> MTTFNYTNILTQAVDELSESQSYKGLFHQHKDGDPLPSAKSLYKIVELARAIIFPGYFGNSTVNSHTINYHIGVNVETLFGLLTEQILAGLCFGQENSKNATDDNEPCRETASLLAARFISKLPELRRILATDVEAAYYGDPAATCFGEIISCYPAIRAISNYRIAHELLILGVPLIPRFITEMAHSETGIDIHPGAQIGHHFTIDHGTGVVIGATSIIGNNVKLYQG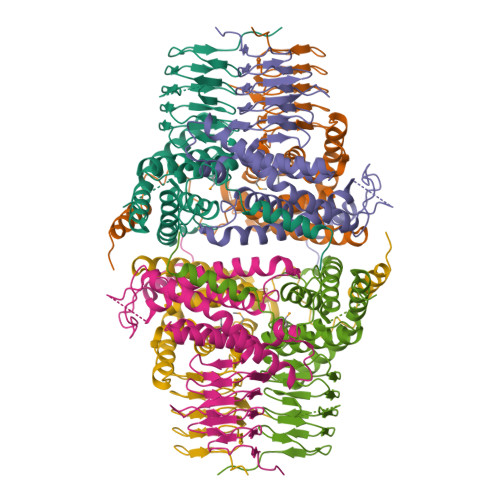VTLGAKSFPLDNNGNPIKGIPRHPILEDDVIVYSNATILGRVTIGKGATVGGNIWVTENVPAGSRIVQRKNKDELEHHHHHH> MDALESLLDEVALEGLDGLCLPALWSRLETRVPPFPLPLEPCTQEFLWRALATHPGISFYEEPRERPDLQLQDRYEEIDLETGILESRRDPVALEDVYPIHMILENKDGIQGSCRYFKERKNITNDIRTKSLQPRCTMVEAFDRWGKKLIIVASQAMRYRALIGQEGDPDLKLPDFSYCILERLGRSRWQGELQRDLHTTAFKVDAGKLHYHRKILNKNGLITMQSHVIRLPTGAQQHSILLLLNRFHVDRRSKYDILMEKLSVMLSTRTNHIETLGKLREELGLCERTFKRLYQYMLNAGLAKVVSLRLQEIHPECGPCKTKKGTDVMVRCLKLLKEFKRNDHDDDEDEEVISKTVPPVDIVFERDMLTQTYDLIERRGTKGISQAEIRVAMNVGKLEARMLCRLLQRFKVVKGFMEDEGRQRTTKYISCVFAEESDLSRQYQREKARSELLTTVSLASMQEESLLPEGEDTFLSESDSEEERSSSKRRGRGSQKDTRASANLRPKTQPHHSTPTKGGWKVVNLHPLKKQPPSFPGAAEERACQSLASRDSLLDTSSVSEPNVSFVSHCADSNSGDIAVIEEVRMENPKESSSSLKTGRHSSGQDKPHETYRLLKRRNLIIEAVTNLRLIESLFTIQKMIMDQEKQEGVSTKCCKKSIVRLVRNLSEEGLLRLYRTTVIQDGIKKKVDLVVHPSMDQNDPLVRSAIEQVRFRISNSSTANRVKTSQPPVPQGEAEEDSQGKEGPSGSGDSQLSASSRSESGRMKKSDNKMGITPLRNYHPIVVPGLGRSLGFLPKMPRLRVVHMFLWYLIYGHPASNTVEKPSFISERRTIKQESGRAGVRPSSSGSAWEACSEAPSKGSQDGVTWEAEVELATETVYVDDASWMRYIPPIPVHRDFGFGWALVSDILLCLPLSIFIQIVQVSYKVDNLEEFLNDPLKKHTLIRFLPRPIRQQLLYKRRYIFSVVENLQRLCYMGLLQFGPTEKFQDKDQVFIFLKKNAVIVDTTICDPHYNLARSSRPFERRLYVLNSMQDVENYWFDLQCVCLNTPLGVVRCPRVRKNSSTDQGSDEEGSLQKEQESAMDKHNLERKCAMLEYTTGSREVVDEGLIPGDGLGAAGLDSSFYGHLKRNWIWTSYIINQAKKENTAAENGLTVRLQTFLSKRPMPLSARGNSRLNIWGEARVGSELCAGWEEQFEVDREPSLDRNRRVRGGKSQKRKRLKKDPGKKIKRKKKGEFPGEKSKRLRYHDEADQSALQRMTRLRVTWSMQEDGLLVLCRIASNVLNTKVKGPFVTWQVVRDILHATFEESLDKTSHSVGRRARYIVKNPQAYLNYKVCLAEVYQDKALVGDFMNRRGDYDDPKVCANEFKEFVEKLKEKFSSALRNSNLEIPDTLQELFARYRVLAIGDEKDQTRKEDELNSVDDIHFLVLQNLIQSTLALSDSQMKSYQSFQTFRLYREYKDHVLVKAFMECQKRSLVNRRRVNHTLGPKKNRALPFVPMSYQLSQTYYRIFTWRFPSTICTESFQFLDRMRAAGKLDQPDRFSFKDQDNNEPTNDMVAFSLDGPGGNCVAVLTLFSLGLISVDVRIPEQIIVVDSSMVENEVIKSLGKDGSLEDDEDEEDDLDEGVGGKRRSMEVKPAQASHTNYLLMRGYYSPGIVSTRNLNPNDSIVVNSCQMKFQLRCTPVPARLRPAAAPLEELTMGTSCLPDTFTKLINPQENTCSLEEFVLQLELSGYSPEDLTAALEILEAIIATGCFGIDKEELRRRFSALEKAGGGRTRTFADCIQALLEQHQVLEVGGNTARLVAMGSAWPWLLHSVRLKDREDADIQREDPQARPLEGSSSEDSPPEGQAPPSHSPRGTKRRASWASENGETDAEGTQMTPAKRPALQDSNLAPSLGPGAEDGAEAQAPSPPPALEDTAAAGAAQEDQEGVGEFSSPGQEQLSGQAQPPEGSEDPRGFTESFGAANISQAARERDCESVCFIGRPWRVVDGHLNLPVCKGMMEAMLYHIMTRPGIPESSLLRHYQGVLQPVAVLELLQGLESLGCIRKRWLRKPRPVSLFSTPVVEEVEVPSSLDESPMAFYEPTLDCTLRLGRVFPHEVNWNKWIHLGGGSGGGSGGSLEVLFQGPGSGSDYKDDDDKGDYKDDDDKGDYKDDDDK;> MNTADQARVGPADDGPAPSGEEEGEGGGEAGGKEPAADAAPGPSAAFRLMVTRREPAVKLQYAVSGLEPLAWSEDHRVSVSTARSIAVLELICDVHNPGQDLVIHRTSVPAPLNSCLLKVGSKTEVAECKEKFAASKDPTVSQTFMLDRVFNPEGKALPPMRGFKYTSWSPMGCDANGRCLLAALTMDNRLTIQANLNRLQWVQLVDLTEIYGERLYETSYRLSKNEAPEGNLGDFAEFQRRHSMQTPVRMEWSGICTTQQVKHNNECRDVGSVLLAVLFENGNIAVWQFQLPFVGKESISSCNTIESGITSPSVLFWWEYEHNNRKMSGLIVGSAFGPIKILPVNLKAVKGYFTLRQPVILWKEMDQLPVHSIKCVPLYHPYQKCSCSLVVAARGSYVFWCLLLISKAGLNVHNSHVTGLHSLPIVSMTADKQNGTVYTCSSDGKVRQLIPIFTDVALKFEHQLIKLSDVFGSVRTHGIAVSPCGAYLAIITTEGMINGLHPVNKNYQVQFVTLKTFEEAAAQLLESSVQNLFKQVDLIDLVRWKILKDKHIPQFLQEALEKKIESSGVTYFWRFKLFLLRILYQSMQKTPSEALWKPTHEDSKILLVDSPGMGNADDEQQEEGTSSKQVVKQGLQERSKEGDVEEPTDDSLPTTGDAGGREPMEEKLLEIQGKIEAVEMHLTREHMKRVLGEVYLHTWITENTSIPTRGLCNFLMSDEEYDDRTARVLIGHISKKMNKQTFPEHCSLCKEILPFTDRKQAVCSNGHIWLRCFLTYQSCQSLIYRRCLLHDSIARHPAPEDPDWIKRLLQSPCPFCDSPVF;> MHHHHHHENLYFQGMDTCGVGYVALGEAGPVGNMTVVDSPGQEVLNQLDVKTSSEMTSAEASVEMSLPTPLPGFEDSPDQRRLPPEQESLSRLEQPDLSSEMSKVSKPRASKPGRKRGGRTRKGPKRPQQPNPPSAPLVPGLLDQSNPLSTPMPKKRGRKSKAELLLLKLSKDLDRPESQSPKRPPEDFETPSGERPRRRAAQVALLYLQELAEELSTALPAPVSCPEGPKVSSPTKPKKIRQPAACPGGEEVDGAPRDEDFFLQVEAEDVEESEGPSESSSEPEPVVPRSTPRGSTSGKQKPHCRGMAPNGLPNHIMAPVWKCLHLTKDFREQKHSYWEFAEWIPLAWKWHLLSELEAAPYLPQEEKSPLFSVQREGLPEDGTLYRINRFSSITAHPERWDVSFFTGGPLWALDWCPVPEGAGASQYVALFSSPDMNETHPLSQLHSGPGLLQLWGLGTLQQESCPGNRAHFVYGIACDNGCIWDLKFCPSGAWELPGTPRKAPLLPRLGLLALACSDGKVLLFSLPHPEALLAQQPPDAVKPAIYKVQCVATLQVGSMQATDPSECGQCLSLAWMPTRPHQHLAAGYYNGMVVFWNLPTNSPLQRIRLSDGSLKLYPFQCFLAHDQAVRTLQWCKANSHFLVSAGSDRKIKFWDLRRPYEPINSIKRFLSTELAWLLPYNGVTVAQDNCYASYGLCGIHYIDAGYLGFKAYFTAPRKGTVWSLSGSDWLGTIAAGDISGELIAAILPDMALNPINVKRPVERRFPIYKADLIPYQDSPEGPDHSSASSGVPNPPKARTYTETVNHHYLLFQDTDLGSFHDLLRREPMLRMQEGEGHSQLCLDRLQLEAIHKVRFSPNLDSYGWLVSGGQSGLVRIHFVRGLASPLGHRMQLESRAHFNAMFQPSSPTRRPGFSPTSHRLLPTP

Transcription factor (TF) IIIC, a six-subunit protein complex with a molecular weight (MW) of 624 kDa in humans, facilitates transcription of type 1 (5S ribosomal RNA) and type 2 [e.g., transfer RNAs (tRNAs)] RNA polymerase (Pol) III target genes. TFIIIC is composed of two subcomplexes, τA and τB, that bind two gene internal DNA motifs: A-box and B-box. τA binds the A-box with low affinity and is required to recruit TFIIIB to the promoter DNA. τB interacts with the B-box with high affinity and, therefore, is essential for target DNA recognition of type 2 genes. hTFIIIC consists of τA subunits TFIIIC35, TFIIIC63, and TFIIIC102 and τB subunits TFIIIC90, TFIIIC110, and TFIIIC220. TFIIIC220 forms an integral part of both τA and τB connecting the two subcomplexes via a ~550–amino acid residue flexible linker.

The cryo-EM structure of DNA-bound human τB enabled us to unveil the molecular basis of B-box DNA recognition. The 3.2-Å cryo-EM map of DNA-bound τB was of sufficient quality to assign 35 bp (55 to 89) of the DNA sequence. We could also assign the N-terminal third (1 to 716) of subunit TFIIIC220 (τ138 in yeast) featuring four WH domains and one extended WH (eWH) domain to human τB. The τB module recognizes the B-box via DNA shape and sequence readout through the assembly of multiple winged-helix domains. The first step involves the high-affinity DNA sequence and shape readout of the B-box motif via an assembly cascade of WH domains. WH2 and WH4 of TFIIIC220 are an integral part of the rigid τB-core, formed by TFIIIC90-TFIIIC110 and the TFIIIC220-WH1 domain, and their conformation does not change upon DNA binding, suggesting that they provide the platform for initial DNA recognition. In addition, the TFIIIC-DNA interaction is further stabilized by the WD40 domain in TFIIIC110, which binds the DNA downstream of the B-box via a positively charged groove. Subsequently, the WH3 and eWH domains recognize the upstream half of the B-box, and the WH domains, collectively, enclose the B-box motif and its upstream region. K657 (eWH) binding induces the opening of the DNA major groove and compaction of the corresponding minor groove, whereas R422/Q423 and R401 (WH3) widen the DNA minor groove. Hence, TFIIIC initiates recognition of the tRNA gene promoter in an evolutionary conserved manner via a combined DNA shape and sequence readout of the B-box DNA motif.> SLPEGKIMPNTVFVGGIDVRMDETEIRSFFARYGSVKEVKIITDRTGVSKGYGFVSFYNDVDVQKIVESQINFHGKKLKLGPAIRKQNLSTYHVQPRPLIF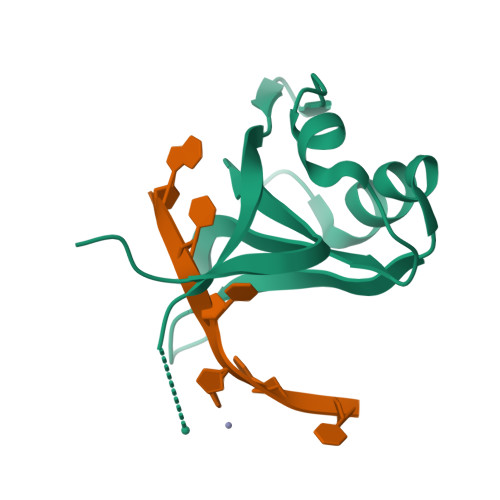N>[2x]MDIGINSDPNSSTQSYKD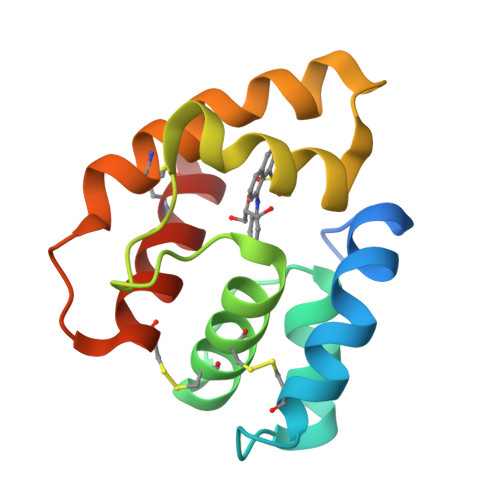AMGPLVRECMGSVSATEDDFKTVLNRNPLESRTAQCLLACALDKVGLISPEGAIYTGDDLMPVMNRLYGFNDFKTVMKAKAVNDCANQVNGAYPDRCDLIKNFTDCVRNSY>MFKIGSVLKQIRQELNYHQIDLYSGIMSKSVYIKVEADSRPISVEELSKFSERLGVNFFEILNRAGMNTKSVNETGKEKLLISKIFTNPDLFDKNFQRIEPKRLTSLQYFSIYLGYISIAHHYNIEVPTFNKTITSDLKHLYDKRTTFFGIDYEIVSNLLNVLPYEEVSSIIKPMYPIVDSFGKDYDLTIQTVLKNALTISIMNRNLKEAQYYINQFEHLKTIKNISINGYYDLEINYLKQIYQFLTDKNIDSYLNAVNIINIFKIIGKEDIHRSLVEELTKI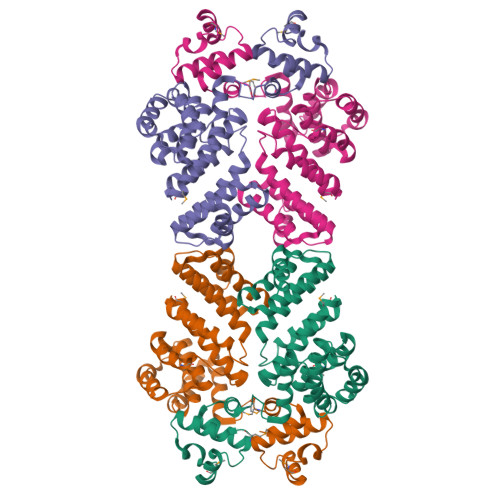SAKEKFTPPKEVTMYYENYVAIENNPIPEIKEQS[12x]> SAQDVDECSLGANPCEHAGKCINTLGSFECQCLQGYT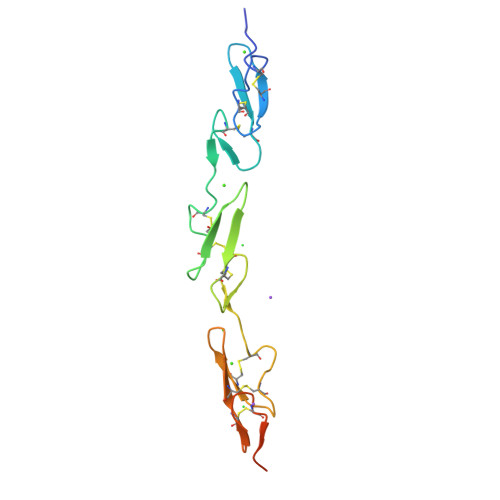GPRCEIDVNECVSNPCQNDATCLDQIGEFQCICMPGYEGVHCEVNTDECASSPCLHNGRCLDKINEFQCECPTGFTGHLCQVDLHHILDAQKMVWNHR>MAAKPVLYYFNGRGKMESIRWLLAAAGVEFEEVFLETREQYEKLLQSGILMFQQVPMVEIDGMKLVQTRAILNYIAGKYNLYGKDLKERALIDMYVGGTDDLMGFLLSFPFLSAEDKVKQCAFVVEKATSRYFPAYEKVLKDHGQDFLVGNRLSWADIHLLEAILMVEEKKSDALSGFPLLQAFKKRISSIPTIKKFLAPGSKRKPISDDKYVETVRRVLR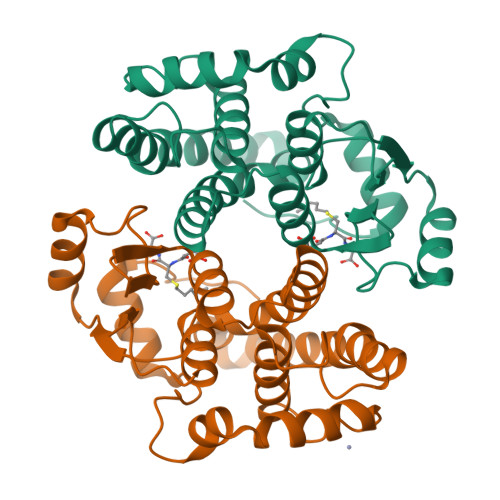MYYDVKPH[2x]> MSNITIYHNPACGTSRNTLEMIRNSGTEPTIILYLENPPSRDELVKLIADMGISVRALLRKNVEPYEQLGLAEDKFTDDQLIDFMLQHPILI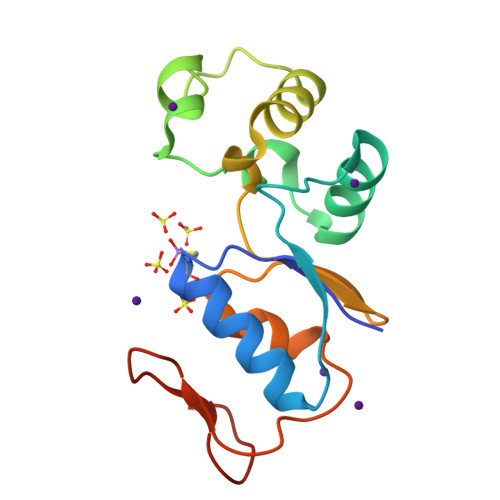NRPIVVTPLGTRLCRPSEVVLDILQDAQKGAFTKEDGEKVVDEAGKRL>MRFKAELMNAPEMRRALYRIAHEIVEANKGTEGLALVGIHTRGIPLAHRIARFIAEFEGKEVPVGVLDITLYRDDLTEIGYRPQVRETRIPFDLTGKAIVLVDDVLYTGRTARAALDALIDLGRPRRIYLAVLVDRGHRELPIRADFVGKNVPTSRSEVVKV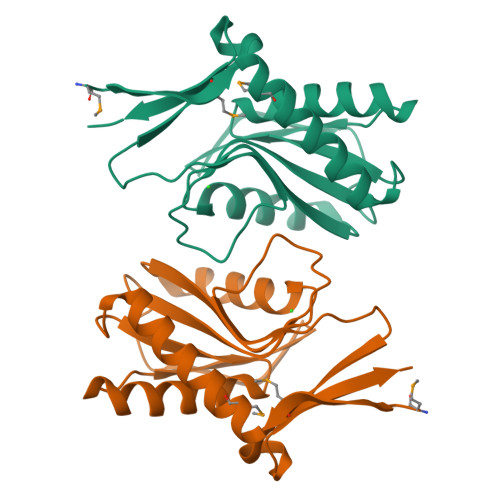KVEEVDGEDRVELWEREGA[4x]>[2x]SMKLTIPELSLVVLIGSSGSGKSTFAKKHFKPTEVISSDFCRGLMSDDENDQTVT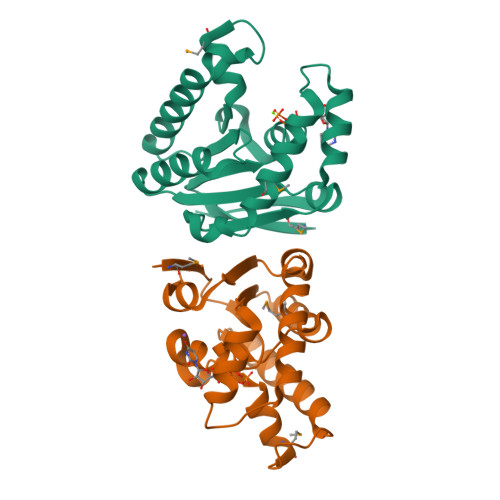GAAFDVLHYIVSKRLQLGKLTVVDATNVQESARKPLIEIAKDYHCFPVAVVFNLPEKVCQERNKNRTDRQVEEYVIRKHTQQMKKSIKGLQREGFRYVYILNSPEEVEEVVFERQP>ANSGEAPKNFGLDVKITGESENDRDLGTAPGGTLNDIGIDLRPWAFGQWGDWSAYFMGQAVAATDTIETDTLQSDTDDGNNSRNDGREPDKSYLAAREFWVDYAGLTAYPGEHLRFGRQRLREDSGQWQDTNIEALNWSFETTLLNAHAGVAQRFSE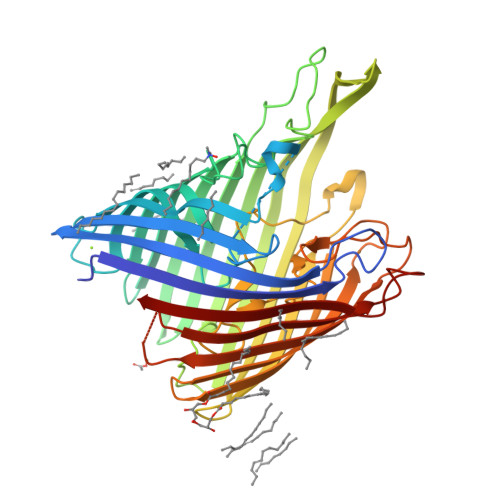YRTDLDELAPEDKDRTHVFGDISTQWAPHHRIGVRIHHADDSGHLRRPGEEVDNLDKTYTGQLTWLGIEATGDAYNYRSSMPLNYWASATWLTGDRDNLTTTTVDDRRIATGKQSGDVNAFGVDLGLRWNIDEQWKAGVGYARGSGGGKDGEEQFQQTGLESNRSNFTGTRSRVHRFGEAFRGELSNLQAATLFGSWQLREDYDASLVYHKFWRVDDDSDIGTSGINAALQPGEKDIGQELDLVVTKYFKQGLLPASMSQYVDEPSALIRFRGGLFKPGDAYGPGTDSTMHRAFVDFIWRF[2x]>[4x]MASQTITVGPWGGPGGNEWDDGSYTGIRIIELSYKEAIGSFSVIYDLNGEPFSGSKHTSKLPYTNVKIELQFPEEFLVSVSGYTAPFSSLATRTPVVRSLKFKTNKGRTFGPYGE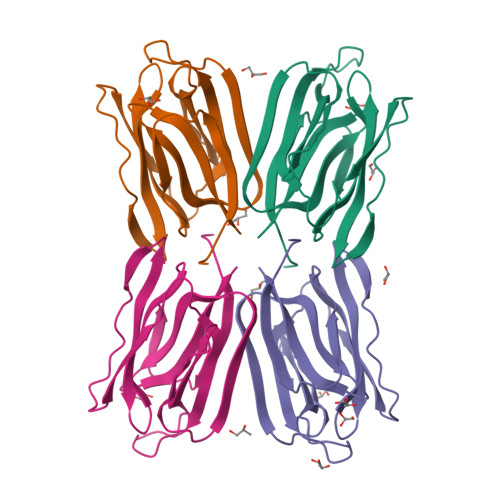EDGTYFNLPIENGLVVGFKGRTGDLLDAIGVHMAL> MDGMKRTELDMYDDIFAVLERFPN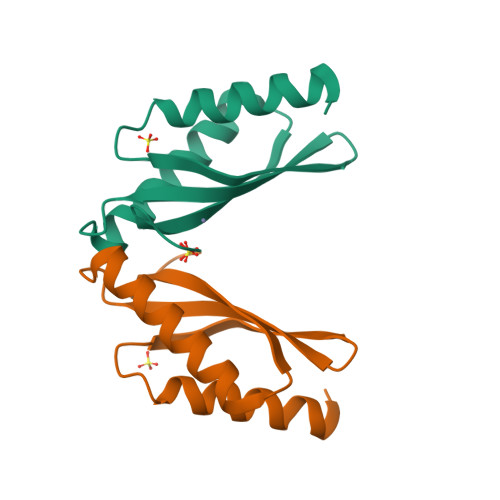VHNPHRVRIRRVGTKYFIEMDIEVDGKMSVKDAHELTVKIRKEMLKRRDDIEDVTIHVEPLGNVEEEGFGLKKGEKK>GSHMSAPLPLDELRTFAEVLDRVKAAYVEPVDDKTLLENAIKGMLSNLDPHSAYLGPEDFAELQESTSGEFGGLGIEVGSEDGFIKVVSPIDDTPAARAGIQPGDLIVQIDGKPTKGQSMTEAVDSMRGKAGSPITLTIVRDGGRPFDVELKRAIIKVKSVKSQVLEPGYAYLRITQFQVNTGEEVVKALNQLRKDNKGRLKGLVLDLRNNPGGVLQSAVEVADAFLTKGLIVYTKGRIANSELRFSADPADPSDKVPLVVLINGGSAAAAEIVAGALQDQKRAILMGTDSFGKGSVQTVLPLNNDRALKLTTALYYTPNGRSIQAQGIVPDIEVGRAKVTQERSSFEGFKEADLQGHLANGNGGADRPTGKRAAPSERPQDSDYQLSQALSLLKGLSVTRGN[6x];>MEDTAVETKAKP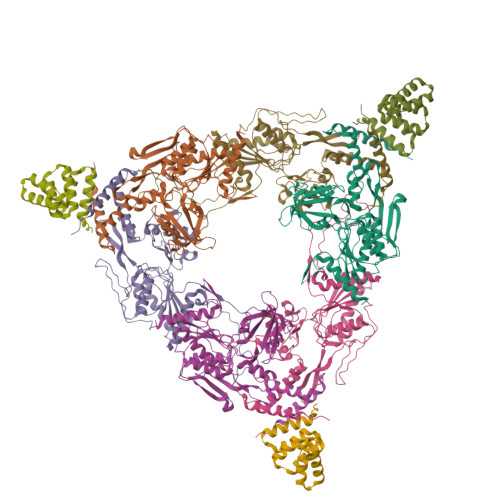EKYGSFSEDSLYSLLVAELAGQRNRFDIALSNYVVQAQKTRDPGVSERAFRIAEYLGADQEALDTSLLWARSAPDNLDAQRAAAIQLARAGRYEESMVYMEKVLNGQGDTHFDFLALSAAETDPDTRAGLLQSFDHLLKKYPNNGQLLFGKALLLQQDGRPDEALTLLEDNSASRHEVAPLLLRSRLLQSMKRSDEALPLLKAGIKEHPDDKRVRLAYARLLVEQNRLDDAKAEFAGLVQQFPDDDDLRFSLALVCLEAQAWDEARIYLEELVERDSHVDAAHFNLGRLAEEQKDTARALDEYAQVGPGNDFLPAQLRQTDVLLKAGRVDEAAQRLDKARSEQPDYAIQLYLIEAEALSNNDQQEKAWQAIQEGLKQYPEDLNLLYTRSMLAEKRNDLAQMEKDLRFVIAREPDNAMALNALGYTLADRTTRYGEARELILKAHKLNPDDPAILDSMGWINYRQGKLADAERYLRQALQRYPDHEVAAHLGEVLWAQGRQGDARAIWREYLDKQPDSDVLRRTIKRLTGAETP[3x]>SNAMAPPPFRPENAIKRADELISVGEKQAALQSLHDFITARRIRWATPSTVEPVVFKFLEIGVELKKGKLLKDGLHQYKKLIQGSTEGLVSVGAVARKFIDLVESKIASEQTRADELQKQEIDDDLEGGVTPENLLISVYESDQSVAGFNDEAITSWLRFTWESYRAVLDLLRNNALLEITYSGVVKKTMHFCLKYQRKNEFKRLAEMLRQHLDAANYQQSKSGNNLVDLSDADTLQRYLDQRFQQVDVSVKLELWHEAYRSIEDVFHLMKISKRAPKPSTLANYYENLVKVFFVSGDPLLHTTAWKKFYKLYSTNPRATEEEFKTYSSTIFLSAISTQLDEIPSIGYDPHLRMYRLLNLDAKPTRKEMLQSIIEDESIYGKVDEELKELYDIIEVNFDVDTVKQQLENLLVKLSSKTYFSQYIAPLRDVIMRRVFVAASQKFTTVSQSELYKLATLPAPLDLSAWDIEKSLLQAAVEDYVSITIDHESAKVTFAKD[3x]

Eukaryotic translation initiation requires the recruitment of the large, multiprotein eIF3 complex to the 40S ribosomal subunit. EIF3 is a large and structurally complex molecular assembly that, in the majority of eukaryotes, consists of 11–13 subunits (eIF3a-eIF3m) with a molecular weight of 600–800 kDa. We present X-ray structures of all major components of the minimal, six-subunit Saccharomyces cerevisiae eIF3 core. Yeast eIF3 engages 40S in a clamp-like manner, fully encircling 40S to position key initiation factors on opposite ends of the mRNA channel, providing a platform for the recruitment, assembly, and regulation of the translation initiation machinery.

The structure of the full-length PCI domain of eIF3a (S. cer. residues 1–496) was solved by single-wavelength anomalous dispersion (SAD) with selenomethionine (Se-Met)-labeled protein to a resolution of 3.3 Å. As observed in a truncated structure of eIF3a and in previously characterized PCI modules (Ellisdon and Stewart, 2012; Khoshnevis et al., 2014), the WHD is structurally similar to other PCI proteins, whereas the N-terminal domain has a series of distinct, flatly arranged helical repeats. The positioning of these helices is reminiscent of the concertina-like arrangement of tetratricopeptide repeats (TPR), although, as in other PCI proteins, TPR-like sequence elements are not detectable. Unlike other PCI HDs, which typically have a significant right-handed superhelical twist, eIF3a has two distinct segments to its repeat. Whereas helices 10–14 have a right-handed pitch, helices 1–9 are arranged along a flat plane that is distinct from other PCI proteins with extended helical repeats. PCI modules are characterized by an N-terminal helical domain (HD) and a C-terminal winged helix domain (WHD), which mediates PCI dimerization (Ellisdon et al., 2012).> KISLLPPVNFTIKVTGLAQVLLQWKPNPDQEQRNVNLEYQVKINAPKEDDYETRITESKAVTILHKGFSASVRTILQNDHSLLASSWASAELHAPPGSPGTSIVNLTCTTNTTEDNYSRLRSYQVSLHCTWLVGTDAPEDTQYFLYYRYGSWTEECQEYSKDTLGRNIACWFPRTFILSKGRDWLAVLVNGSSKHSAIRPFDQLFALHAIDQINPPLNVTAEIEGTRLSIQWEKPVSAFPIHCFDYEVKIHNTRNGYLQIEKLMTNAFISIIDDLSKYDVQVRAAVSSMCREA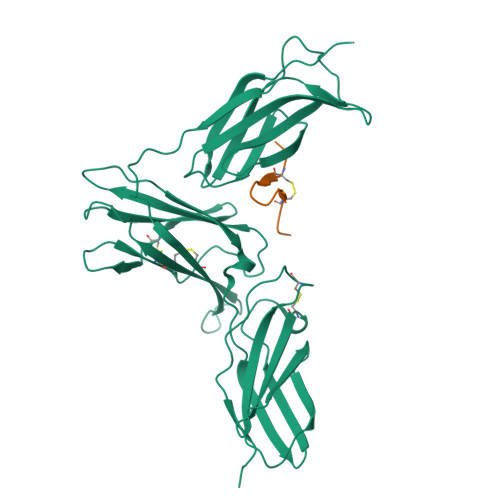GLWSEWSQPIYVGFSR;> VDECWRIIASHTWFCAEE>QDSTSDLIPAPPLSKVPLQQNFQDNQFQGKWYVVGLAGNAILREDKDPQKMYATIYELKEDKSYNVTSVLFRKKKCDYWIRTFVPGSQPGEFTLGNIKSYPGLTSYLVRVVSTNYNQHAMVFFKKVSQNREYFKI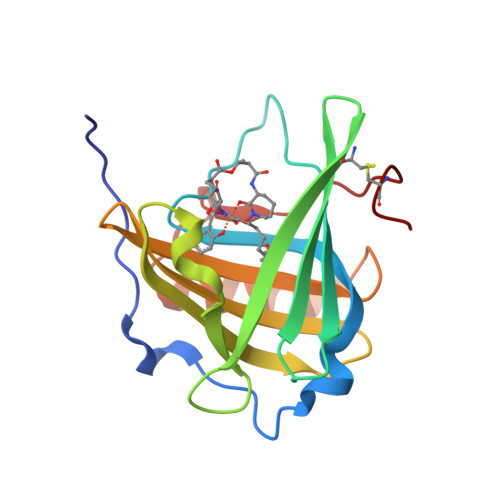TLYGRTKELTSELKENFIRFSKSLGLPENHIVFPVPIDQCIDG[3x]>VEVKIGITDSPRELVFSSAQTPSEV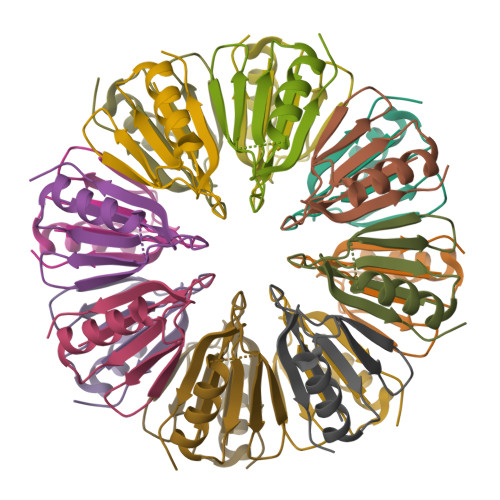EELVSNALRDDSGLLTLTDERGRRFLIHTARIAYVEIGVADARRVGFGVGVDAAAGSAGKVATSG[4x]Here, we report cryo-EM structures of ELIC in liposomes where the ion channel is confirmed to be in resting, activated, and desensitized states. The structures of ELIC in liposomes have the same overall architecture as structures of ELIC or other pLGICs in nanodiscs, consisting of a homopentameric assembly around a central ion conduction pore. Each subunit consists of an ECD and TMD. Proteoliposomes were formed using a 2:1:1 molar ratio of POPC (1-palmitoyl-2-oleoyl-phosphatidylcholine):POPE (1-palmitoyl-2-oleoyl-phosphatidylethanolamine):POPG (1-palmitoyl-2-oleoyl-phosphatidylglycerol); these lipids are known to support ELIC activity, and phosphatidylethanolamine and phosphatidylglycerol are the two principal phospholipids found in gram-negative bacteria in which ELIC is expressed.

To test this possibility, we reconstituted WT ELIC in spNW25, a circularized nanodisc with an average diameter of 25 nm, for single particle cryo-EM analysis, and determined a structure of ELIC in the presence of agonist (propylamine). spNW25 nanodiscs are significantly larger than the 11 nm (spMSP1D1) and 15 nm (spNW15) nanodiscs previously used for agonist-bound WT ELIC structures. Initial inspection of the micrographs showed multiple ELIC particles in most nanodiscs and localization of the particles to the rim of the nanodisc. Consistent with this observation, side views of the 2D class averages and the resulting 3D reconstruction using C1 symmetry showed significant MSP density on one side of the TMD. A C5 reconstruction of agonist-bound WT ELIC in spNW25 also did not show densities for M4. Unexpectedly, the structure in the largest nanodisc, spNW25, deviates most from the liposome structure. In the spNW25 structure, there is a shortening of M1 and M2 and tilting of M3 toward the membrane that decreases the height of these transmembrane helices along the pore axis by ~1–1.5 Å compared to the liposome and spMSP1D1 structures. Along with this, M2 is tilted toward the pore axis, narrowing the pore even further at L240 (9’) and Q233 (2’). Contrary to what was previously suggested, the agonist-bound WT ELIC structure in a large nanodisc (spNW25) deviates most from the structure in liposomes, indicating that such large nanodiscs do not recapitulate the membrane environment of a liposome. Strikingly, ELIC localizes only to the rim of this large nanodisc.

>[5x]APADNAADARPVDVSVSIFINKIYGVNTLEQTYKVDGYIVAQWTGKPRKTPGDKPLIVENTQIERWINNGLWVPALEFINVVGSPDTGNKRLMLFPDGRVIYNARFLGSFSNDMDFRLFPFDRQQFVLELEPFSYNNQQLRFSDIQVYTENIDNEEIDEWWIRGKASTHISDIRYDHLSSVQPNQNEFSRITVRIDAVRNPSYYLWSFILPLGLIIAASWSVFWLESFSERLQTSFTLMLTVVAYAFYTSNILPRLPYTTVIDQMIIAGYGSIFAAILLIIFAHHRQANGVEDDLLIQRCRLAFPLGFLAIGCVLVIRGITL>SNAEDELYRQSLEIISRYLREQATGAKDTKPMGRSGATS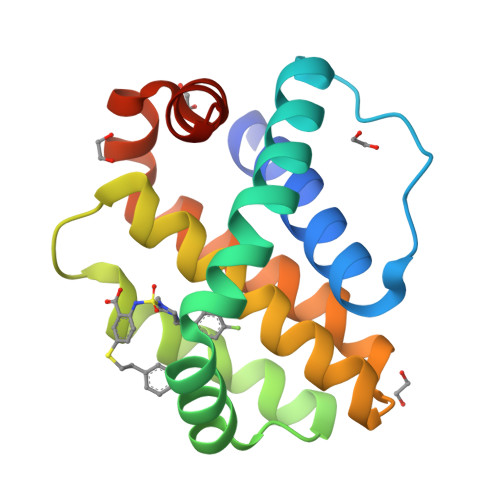RKALETLRRVGDGVQRNHETAFQGMLRKLDIKNEDDVKSLSRVMIHVFSDGVTNWGRIVTLISFGAFVAKHLKTINQESCIEPLAESITDVLVRTKRDWLVKQRGWDGFVEFFHVED[4x]>MADPWQECMDYAVILARQAGEMIREALKNEMDVMIKSSPADLVTVTDQKVEKMLMSSIKEKYPCHSFIGEESVAAGEKTVFTEQPTWVIDPIDGTTNFVHRFPFVAVSIGFLVNKEMEFGIVYSCVEDKMYTGRKGKGAFCNGQKLQVSQQEDITKSLLVTELGSSRKPETLRIVLSNMEKLCSIPIHGI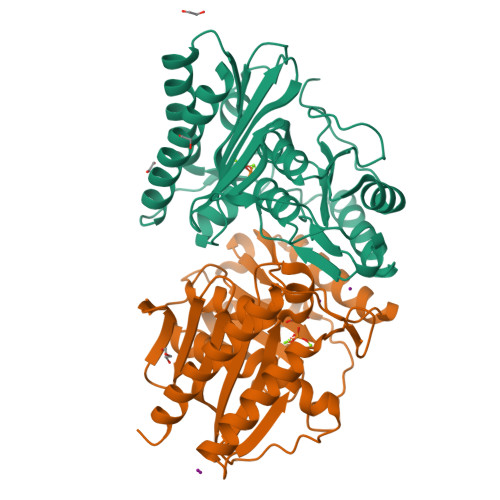RSVGTAAVNMCLVATGGADAYYEMGIHCWDMAGAGIIVTEAGGVLMDVTGGPFDLMSRRIIAANSITLAKRIAKEIEIIPLQRDDES[4x]>[4x]MSFEGARLSMRSRRNGTMGSTRTLYSSVSRSTDVSYSDSDLVNFIQANFKKRECVFFTRDSKAMENICKCGYAQSQHIEGTQINQNEKWNYKKHTKEFPTDAFGDIQFETLGKKGKYLRLSCDTDSETLYELLTQHWHLKTPNLVISVTGGAKNFALKPRMRKIFSRLIYIAQSKGAWILTGGTHYGLMKYIGEVVRDNTISRNSEENIVAIGIAAWGMVSNRDTLIRSCDDEGHFSAQYIMDDFTRDPLYILDNNHTHLLLVDNGCHGHPTVEAKLRNQLEKYISERTSQDSNYGGKIPIVCFAQGGGRETLKAINTSVKSKIPCVVVEGSGQIADVIASLVEVEDVLTSSMVKEKLVRFLPRTVSRLPEEEIESWIKWLKEILESSHLLTVIKMEEAGDEIVSNAISYALYKAFSTNEQDKDNWNGQLKLLLEWNQLDLASDEIFTNDRRWESADLQEVMFTALIKDRPKFVRLFLENGLNLQKFLTNEVLTELFSTHFSTLVYRNLQIAKNSYNDALLTFVWKLVANFRRSFWKEDRSSREDLDVELHDASLTTRHPLQALFIWAILQNKKELSKVIWEQTKGCTLAALGASKLLKTLAKVKNDINAAGESEELANEYETRAVELFTECYSNDEDLAEQLLVYSCEAWGGSNCLELAVEATDQHFIAQPGVQNFLSKQWYGEISRDTKNWKIILCLFIIPLVGCGLVSFRKKPIDKHKKLLWYYVAFFTSPFVVFSWNVVFYIAFLLLFAYVLLMDFHSVPHTPELILYALVFVLFCDEVRQWYMNGVNYFTDLWNVMDTLGLFYFIAGIVFRLHSSNKSSLYSGRVIFCLDYIIFTLRLIHIFTVSRNLGPKIIMLQRMLIDVFFFLFLFAVWMVAFGVARQGILRQNEQRWRWIFRSVIYEPYLAMFGQVPSDVDSTTYDFSHCTFSGNESKPLCVELDEHNLPRFPEWITIPLVCIYMLSTNILLVNLLVAMFGYTVGIVQENNDQVWKFQRYFLVQEYCNRLNIPFPFVVFAYFYMVVKKCFKCCCKEKNMESNACCFRNEDNETLAWEGVMKENYLVKINTKANDNSEEMRHRFRQLDSKLNDLKSLLKEIANNIKLEGGSSGGWSHPQFEK

Transient receptor potential melastatin 8 (TRPM8) channel is a Ca2+-permeable non-selective cation channel that acts as the primary cold sensor in humans. TRPM8 is also activated by ligands such as menthol, icilin, and phosphatidylinositol 4,5-bisphosphate (PIP2), and desensitized by Ca2+. MmTRPM8 is a homotetramer with dimensions of 140 × 110 × 110 Å. Each MmTRPM8 subunit contains multiple domains, including the N-terminal four TRPM homology repeats (MHR1 to MHR4), S1–S6 six transmembrane helices in a domain swap configuration, TRP helix, and C-terminal coiled-coil.

We first determined MmTRPM8 structures in the detergent Lauryl Maltose Neopentyl Glycol (LMNG) in the absence of ligand at 3.0 Å resolution (MmTRPM8LMNG-ligand-free), and in the presence of Ca2+ at 2.9 Å resolution (MmTRPM8LMNG-Ca), Ca2+ + icilin at 3.0 Å resolution (MmTRPM8LMNG-Ca-icilin), and Ca2+ + icilin + PIP2 at 3.2 Å resolution (MmTRPM8LMNG-Ca-icilin-PIP2). In the map of MmTRPM8LMNG-Ca, strong density shows that a Ca2+ ion is harbored by the cytosolic-facing cavity in the VSLD. The Ca2+ is coordinated by side chains of residues Glu782, Gln785, Asn799, and Asp802 from S2 and S3. In addition, the side chain of Tyr793 from the S2-S3 linker is positioned in proximity. To confirm this Ca2+ binding site in MmTRPM8, we performed all-atom molecular dynamic (MD) simulations using the Ca2+-bound structure MmTRPM8LMNG-Ca as an initial model. Throughout 250 ns simulations, the Ca2+ binds stably at this site, with a Root Mean Square Deviation (RMSD) within 3 Å. The distances between Ca2+ and CG atoms of its coordinating residues Glu782, Asn799, and Asp802 remain 2–5 Å in most time of the simulations. Thus, the simulation results support the binding of one Ca2+ ion in this cytosolic-facing cavity in the VSLD of MmTRPM8. Therefore, it is likely that PmTRPM8Ca is also in the closed state, similar to the Ca2+-bound MmTRPM8LMNG-Ca structure.>MRGSHHHHHHTDPALRAMATLLQLHFAFNGPFGDAMAEQLKPLAESINQEPGFLWKVWTESEKNHEAGGIYLFTDEKSALAYLEKHTARLKNLGVEEVV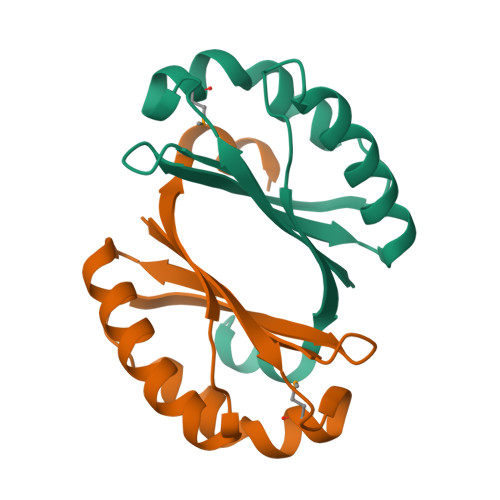AKVFDVNEPLSQINQAKLAGLCGR[2x]>MFEARLVQGSILKKVLEALKDLINEACWDISSSGVNLQSMDSSHVSL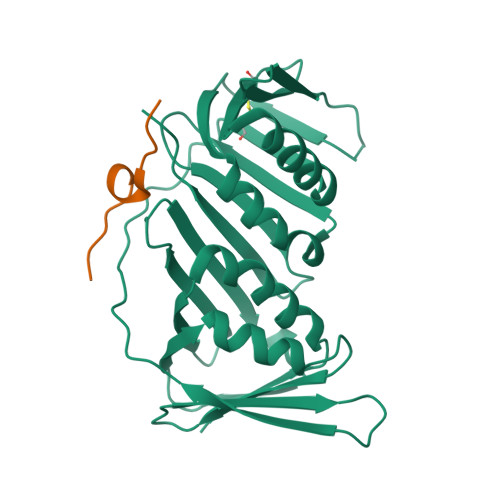VQLTLRSEGFDTYRCDRNLAMGVNLTSMSKILKCAGNEDIITLRAEDNADTLALVFEAPNQEKVSDYEMKLMDLDVEQLGIPEQEYSCVVKMPSGEFARICRDLSHIGDAVVISCAKDGVKFSASGELGNGNIKLSQTSNVDKEEEAVTIEMNEPVQLTFALRYLNFFTKATPLSSTVTLIMSADVPLVVEYKIADMGHLKYYLAPKIEDEEGS[2x];>[2x]STQGRLDDFFKVTGSL> MGHHHHHHAENLYFQGHMHKVKLAAITCELPARSYENDDPVFAAVPDLSESWWQFWGVNRRGYFDPRNGENEFSLVVRAAERLLRSSDTAPDSVDMLICSASSPIMTDAGDVLPDLRGRLYPRMANVLSKQLGLSRALPLDSQMECASFLLNLRLAASMIRQGKAEKVLVVCSEYISNLLDFTSRTSTLFADGCAVALLTRGDDDSCDLLASAEHSDATFYEVATGRWRLPENPTGEAKPRLYFSLFSDGQNKMASFVPTNVPIAMRR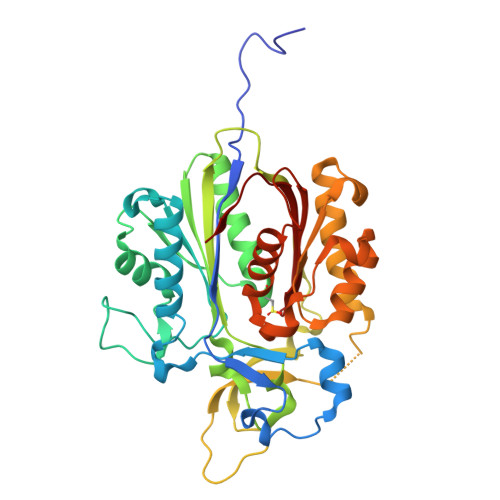ALEKAGLGSDDIDYFVFHQPAPFLVKAWAEGIGARPEQYQLTMGDTGVMISVSIPYTLMTGLREGKIRPGDRIVMAGAATGWGFAAQVWQLGEVLVC>SSKEVAELKKQVESAELKNQRLKEVFQTKI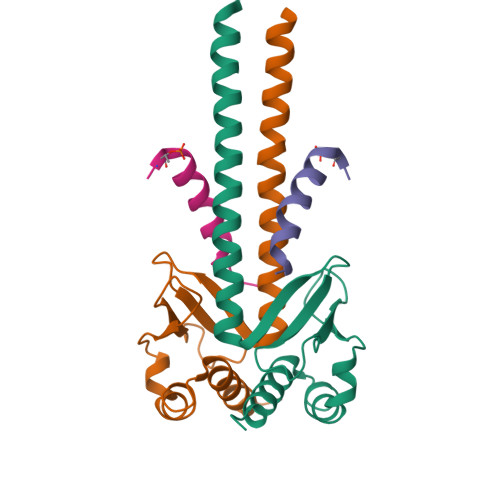QEFRKACYTLTGYQIDITTENQYRLTSLYAEHPGDCLIFKATSPSGSKMQLLETEFSHTVGELIEVHLRRQDSIPAFLSSLTLELFSRQTVA[4x];>KVQPSPTVHTKEALGFIMNMFQAPTS[4x]(3~{Z},6~{S})-3-(1~{H}-imidazol-4-ylmethylidene)-6-propan-2-yl-piperazine-2,5-dione | C11 H14 N4 O2 | 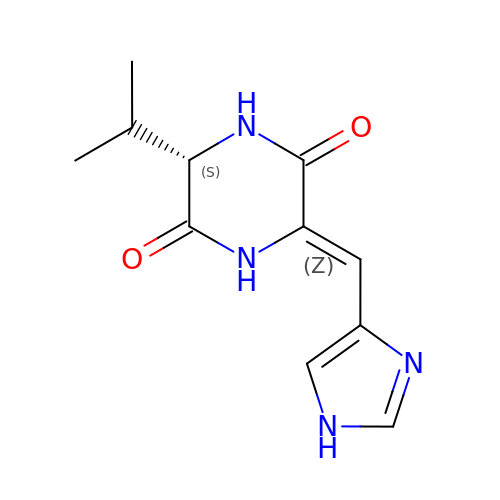VFDJEJCELMPUBS-CHDHTGKKSA-N6-(HYDROXYETHYLDITHIO)-8-(AMINOMETHYLTHIO)OCTANOIC ACID | C11 H23 N O3 S3 | 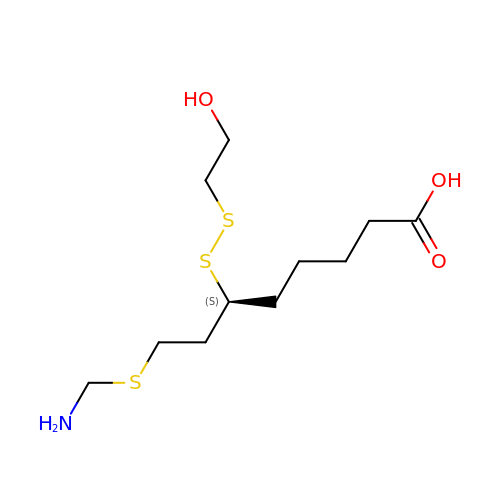BFRWEULQQALYNZ-JTQLQIEISA-N(1R,3S,4R)-1-azabicyclo[2.2.2]octan-3-yl {2-[2-(4-fluorophenyl)-1,3-thiazol-4-yl]propan-2-yl}carbamate 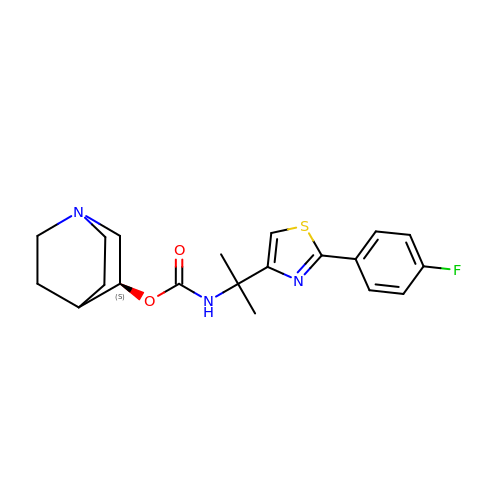| C20 H24 F N3 O2 S | YFHRCLAKZBDRHN-MRXNPFEDSA-N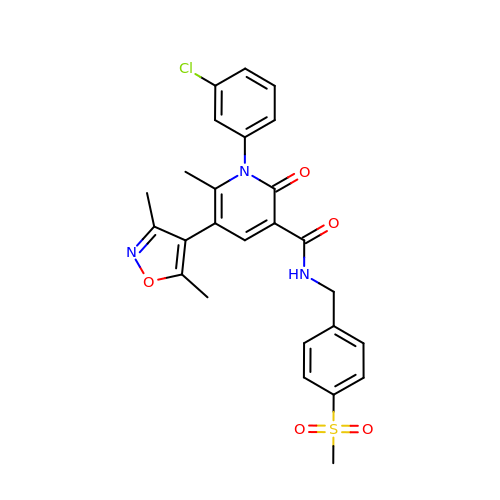1-(3-CHLOROPHENYL)-5-(3,5-DIMETHYLISOXAZOL-4-YL)-6-METHYL-N-[4-(METHYLSULFONYL)BENZYL]-2-OXO-1,2-DIHYDROPYRIDINE-3-CARBOXAMIDE | C26 H24 Cl N3 O5 S | QYWSDDYRNPGJNA-UHFFFAOYSA-N Correct folding of the Lpt system component LptD is regulated by a periplasmic metalloprotease, BepA. Among the LptD quality control proteases, BepA is different in that it also has chaperone activities and influences the insertion of other OMPs into the outer membrane, and its deletion renders cells sensitive to multiple antibiotics. The primary sequence of BepA indicates that this protein is a member of the M48 family of zinc metalloproteases, of which there are four in E. coli. In addition to the N-terminal M48 protease domain, BepA has a C-terminal tetratricopeptide repeat (TPR) domain.

The structure revealed the TPR domain, consisting of 12 α-helices forming 4 TPR motifs and four non-TPR helices, in tight association with the M48 zinc-metallopeptidase domain. This forms a nautilus-like fold with the TPR subdomain cupping the metallopeptidase domain. Helices 8 and 9 contribute a tight turn at the end of the TPR domain, allowing the M48 metallopeptidase domain to be cupped by the pocket formed from TPR motifs 2 and 3. Interaction of the protease domain with the TPR pocket creates a larger negatively charged pocket, which is also noted in the structure presented by Shahrizal et al.. The protease domain of BepA consists of the active site α-helix H4 containing the HEXXH motif, and an active-site plug formed by a loop between helices H6 and H7, residues S246 to P249. The active-site zinc ion is coordinated by H136 and H140 within the HEXXH motif, E201 contributed by helix H5, and H246 on a loop that forms the small α-helical active-site plug. Coordination of the zinc ion by H246 acts as the fourth ligand, therefore suggesting that a rearrangement of the active-site plug should be required for proteolytic activity. We did not observe any density corresponding to positions L146 to I194, and considering that this section is in close proximity to the active site, we expect that it may form a dynamic regulatory region. The importance of residue H246 for BepA function, and the conformation of the active-site plug observed in our crystal structure, suggests that the solved crystal structure may represent a proteolytically inactive form of the protein.

> MFRQLKKNLVATLIAAMTIGQVAPAFADSADTLPDMGTSAGSTLSIGQEMQMGDYYVRQLRGSAPLINDPLLTQYINSLGMRLVSHANSVKTPFHFFLINNDEINAFAFFGGNVVLHSALFRYSDNESQLASVMAHEISHVTQRHLARAMEDQQRSAPLTWVGALGSILLAMASPQAGMAALTGTLAGTRQGMISFTQQNEQEADRIGIQVLQRSGFDPQAMPTFLEKLLDQARYSSRPPEILLTHPLPESRLADARNRANQMRPMVVQSSEDFYLAKARTLGMYNSGRNQLTSDLLDEWAKGNVRQQRAAQYGRALQAMEANKYDEARKTLQPLLAAEPGNAWYLDLATDIDLGQNKANEAINRLKNARDLRTNPVLQLNLANAYLQGGQPQEAANILNRYTFNNKDDSNGWDLLAQAEAALNNRDQELAARAEGYALAGRLDQAISLLSSASSQVKLGSLQQARYDARIDQLRQLQERFKPYTKM>GHMKISRETLHQLIENKLCQAGLKREHAATVAEVLVYADARGIHSHGAVRVEYYAERISKGGTNREPEFRLEETGPCSAILHADNAAGQVAAKMGMEHAIKTAQQNGVAVVGISRMGHSGAISYFVQQAARAGFIGISMCQSDPMVVPFGGAEIYYGTNPLAFAAPGEGDEILTFDMATTVQAWGKVLDARSRNMSIPDTWAVDKNGVPTTDPFAVHALLPAAGPKGYGLMMMIDVLSGVLLGLPFGRQVSSMYDDLHAGRNLGQLHIVINPNFFSSSELFRQHLSQTMRELNAITPAPGFNQVYYPGQDQDIKQRKAAVEGIEIVDDI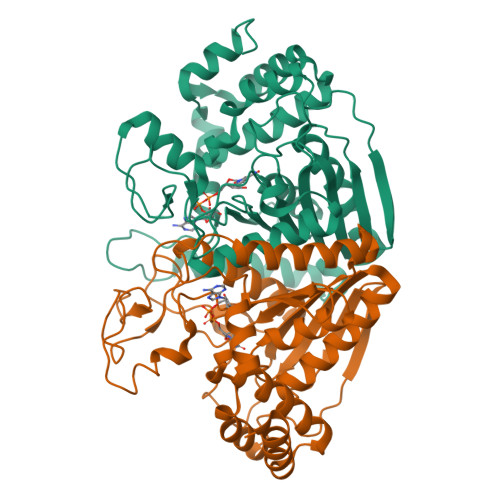YQYLISDALY[2x]> SH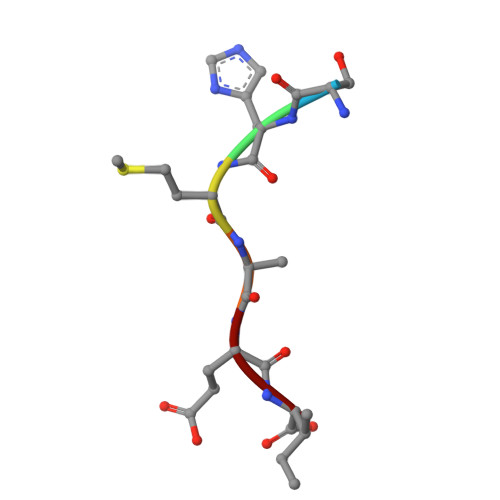MAEI[(2R,5S)-5-(4-amino-5-fluoro-2-oxo-3,6-dihydropyrimidin-1(2H)-yl)-1,3-oxathiolan-2-yl]methyl trihydrogen diphosphate | C8 H14 F N3 O9 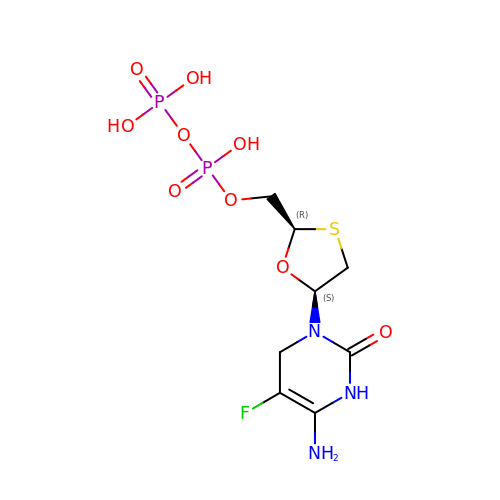P2 S | DSUZHKWUVJBGFZ-NTSWFWBYSA-N> MDKINLVCGSLLHNIGKIIYRGTSERAKHSKLGGDFIKSFEQFRNTELTDCIRYHHAQEITSVKSNKEKN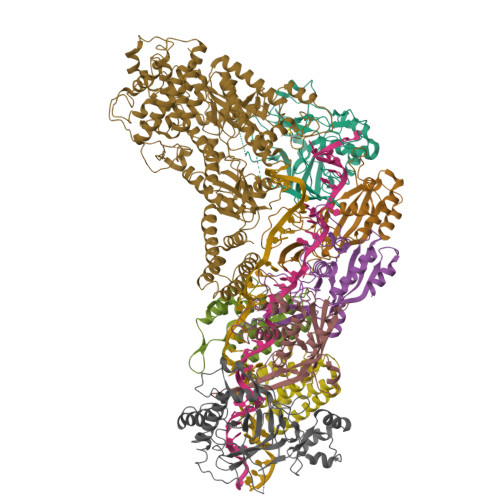SLFYITYIADNISSGMDRRKDLEEGAEGFNWDKKVALGSVFNVLNEKEKGRQNYSYPFVARTRIKEEPLNFPTATQNQYTTSYYDGLITDMKTILQRLKPDKEHINSLLQMMESLWSYVPSSTDKNQLVDISLYDHSRTTAAIASAIYDYFQAENITDYQKELFDYNATEFYDKNAFLMMNFDMSGVQNFIYNISGSKALKSLRARSFYLDMLLEYISDNLLEKLELSRANILYVGGGHAYLLLANTNKTKAILSDFEHDLKTWFLDKFKIDLYVAMAYTEVSANDLMNHNGHYRDIYRRLSQKTSAKKANRYTAEEILNLNHQGTENARECRECKRSDLLIEEDDICEICDSLQKVSRDLTRENIFVIANEGVLDMPFGKKMSALSYSQADKLKKSNAEVQIYAKNISEIGQNLMTRIDMGDYTYRSDFHEMLEEVEVGINRLGVLRADVDNLGQAFINGIPDDYLSISRTATFSRAMSRFFKNYLNQLLAEKSYKINVIYAGGDDLFMIGAWQDILDFSIVLKQKFADFTQNKLSISAGIGMFREKYPVARMASLTGDLEDAAKDYKPDERAVQATKNAVTLFDATNVFSWDTLENDIFVKLDAITKNFEKLDETGKAFIYRLIDLLRGVNENQQINIARLAYTLSRMEEKIGKTFAQELYNWANADRKTLIMALEIYILKTRE;> MKIIKLYFESPVHFGEKRLSESKITFSADTLFSALMIEAVGLGKEDEFYQLASNNLVKFSDAFPFIDQYYYIPKPMFNLKLEKEDENPSKAFKKLLYVPIDSLEDYLSGGLDAYFERESFNLGKLALSEKVQQHDFKDSEPYNVGTFTFKENTGLYVLIEQTHPLLEELLENLQYSGIGGKRNSGYGKFKFEILEDSDIEDLFSAKGNRKILLSGALPKDAELEQALKNASYLLERRGGFVQSDTYATNLVKKQDLYVFKSGSTFENSFDGDIYQVGKKGNHPVYKYAKSFFLEVS;>[2x]TELKIGNEKVNSTNFGDFAEKAIRGINHKPFVNSKGGEQKITTSKIRGILELVNKVYNRVINTNDVELSENILADIAYIKVKIAYESGREPVVKDFIQRTAFTAAITDVMNQRTRESFLLFARYVESLIAYFKFYGGKD;>[3x]MKLVIEGTIVLKTGMHIGGSSDFSAIGAVASPVVRDTLTRLPLIPGSSLKGKMRYLLAKELNNGILLNEPNNDQDEILRLFGSSEKDKIRRARLKFNDIKLSNLAELETFNVSSTEVKFENTINRKTAVANPRQIERVIAGSKFDFEIFYNLDDIKEVEKDFENIKQGFDLLEFDYLGGHGTRGSGRIAFENLSVITAVGNFEKINTLNEILGA;> MKKTYRVTLTALGPIFIGGGEKLKKYEYIFDKQKKVAHMIDHTKFTKYLLEKNLLDDFTSRVNSHFDLYDYLVNKKGIVFMPLVKYSVPVAQFRTEVKNRFGKPISSPPMNDLNTFVKDAFGRPYIPGSSLKGALRTAILNDLKEDTKENEVFAHLQVSDSETIDLENLKVYQKVDYSKTAKPLPLYRECLKPNTEITFTVSFDDEYLTLKKIQNALHKTYQHYYIKWLKGGKVGETLIKGVYDSHADELKKNTFALDQPSQNQGEIIYIGGGAGFVSKTLHYKSKNRDQARNDSFDILKQLFRTTYSKMRSVPDNVPVALKLAVETKTFNGRVTGKHYLEMGKARIKLEEL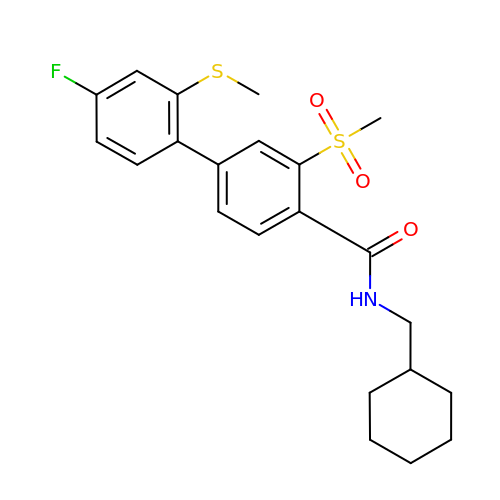~{N}-(cyclohexylmethyl)-4-(4-fluoranyl-2-methylsulfanyl-phenyl)-2-methylsulfonyl-benzamide | C22 H26 F N O3 S2 | SQLMHOPYTBPHSH-UHFFFAOYSA-N> GSHMQDPEQLKHCNGILSELLSSKHAAYAWPFYKPVDASALGLHDYHDIIKH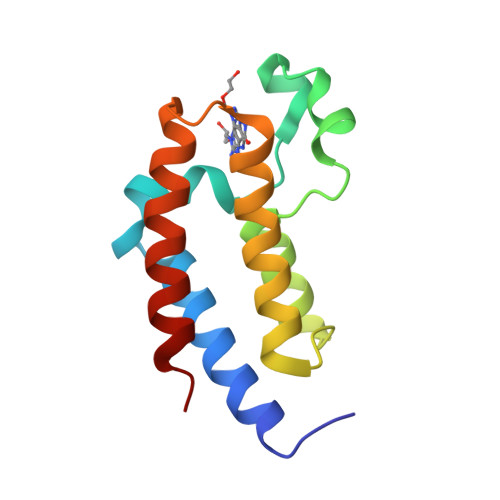PMDLSTVKRKMENRDYRDAQEFAADVRLMFSNCYKYNPPDHDVVAMARKLQDVFEFRYAKMPD>[2x]MADVDELEDPMEEMTSYTFARFLRSPETEAFVRNLDRPPQMPAMRFVYLYCLCKQIQEFSGETGFCDFVSSLVQ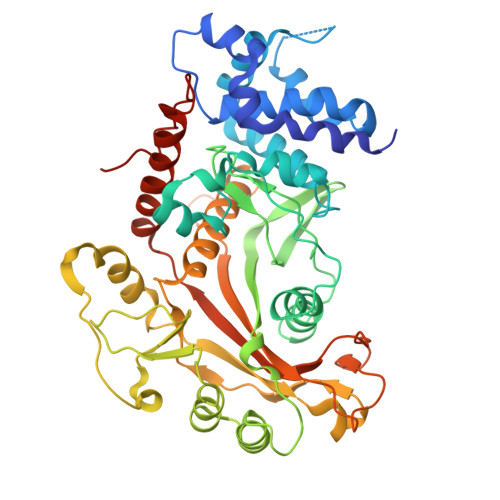ENDSKDGPSLKSIYWGLQEATDEQRTVLCSYVESMTRGQSENLMWDILRNGIISSSKLLSTIKNGPTKVFEPAPISTNHYFGGPVAFGLRCEDTVKDIVCKLICGDASANRQFGFMISPTDGIFGVSLSLCVNVESQGDFILFTDRSCIYEIKCRFKYLFSKSEFDPIYPSYTALYKRPCKRSFIRFINSIARPTVEYVPDGRLPSEGDYLLTQDEAWNLKDVRKRKLGPGHDLVADSLAANRGVESMLYVMTDPSENAGRIGIKDRVPVNIFINPRHNYFYQVLLQYKIVGDYVRHSGGGKPGRDCSPRVNIVTAFFRKRSPLDPATCTLGSDLLLDASVEIPVAVLVTPVVLPDSVIRKTLSTAAGSWKAYADNTFDTAPWVPSGLFADDESTP>MRGSHHHHHHGSQKTSDLIVLGLPWKTTEQDLKEYFSTFGEVLMVQVKKDLKTGHSKGFGFVRFTEYETQVKVMSQRHMIDGRWCDCKLPNSKQSQDEPLRSR[2x]

One example is TDP-43, which binds RNA and DNA and functions in mRNA splicing, translation regulation and transport1. However, when misfolded, TDP-43 aggregates and forms the major component in the ubiquitylated inclusions in the neuronal cells of patients with amyotrophic lateral sclerosis (ALS) and frontotemporal lobar degeneration (FTLD). TDP-43 consists of an N-terminal domain (NTD) and two tandem RNA recognition motifs, RRM1 and RRM2, followed by a C-terminal glycine-rich region (G). It forms homodimers and the two RNA-recognition motifs are involved in nucleic acid binding.

After refinement of the RRM1 domain structure, the difference Fourier map (Fo-Fc) revealed a clear continuous electron density that could be fitted respectively with 8 and 9 nucleotides in the two RRM1/DNA complexes per asymmetric unit. For clarity, only a single RRM1/DNA (chain A) and RRM1-D169G/DNA (chain A) were used for structural presentation and comparison hereafter. Superposition of the RRM1/DNA complexes determined in this and previous studies reveal that the unmodified DNA bound in RRM1 and RRM1-D169G (this study) fit well, but deviate from the Se-labeled DNA around the Se-labeled sites at A5 and G6. The overall structure of RRM1-D169G mutant is similar to that of wild-type RRM1, nevertheless, a small local difference was observed in the β turn (Turn6) containing the D169G mutation. Superposition of the two proteins yielded an average root-mean-square deviation (RMSD) of 0.39 Å for 71 Cα atoms.> QSVKESEGGLFKPTDTLTLTCTASGFSLNGYGVIWVRQAPGKGLEWIGSAGAYGRIYYPNWARSRATITRNTNLNTVSLKMTSLTAADTATYFCARRTNVSTSVGFDSWGPGTLVTVSSSSGQPKAPSVFPLAPCCGDT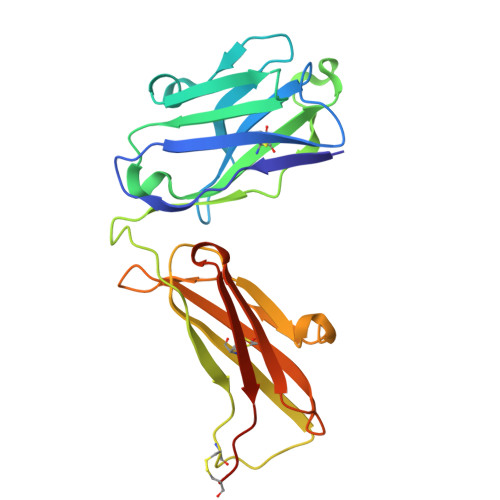PSSTVTLGCLVKGYLPEPVTVTWNSGTLTNGVRTFPSVRQSSGLYSLSSVVSVTSSSQPVTCNVAHPATNTKVDKTVAPSTCSHHHHHH> GPGSMEALVRALEEADHAVATVVQSRILEFFMAAGRETPAGVRGLWARALRLACRAYVETGTCEAAVLAENLAGLALWRLRHDWDEGTAPLLELLGVVNGDDTTAALTEAGLRTSAEFGPDAMFRLVSEWCAAFDEALAGARSADDVLAAPRVVPPEQTARALVQPRFATLYDMDFVQDGLRYVAQHTNWALPLALAVRQMQNEGLKPLTRALFALTIADEFFHDRQNPTLREQFAEAARAVDEAALVPVGEVNATPRTAVEVRVSAALAHGDAYVRELRPGTVARRLRTDQGVLALL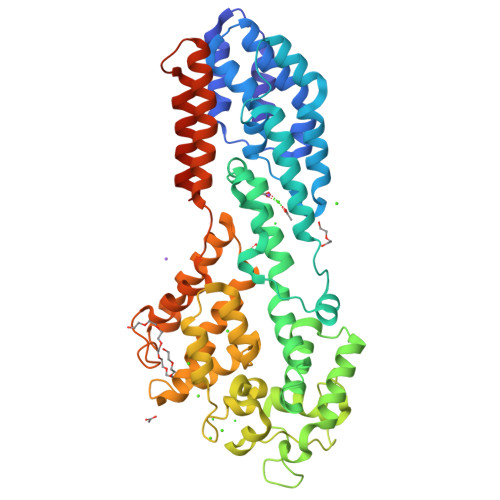DPGAQAVHVAAAADLDHTQVDATGVWEAVAASASPLQVVEALVTAGFTRRHCDLLERAVLDRAPRLTAAQAAVGCTAVVGGVVHRLLDDYGPGLDYVRAYTDVADTLEPLYGDVTAALGLPEKGVEAVVRACMAPRPPTEHVGAARAALLREVAAAERRAGLAHSAAREALNTWLAFRAQSRWGLRADGAGETPMEAPTSAA N6-(penta-2,3-dienyl)adenine | C10 H11 N5 | 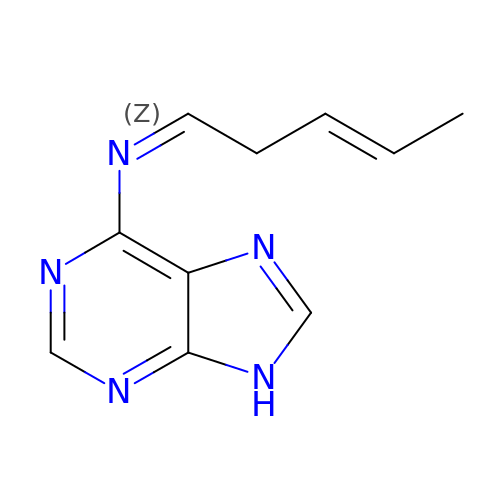ZZNYJUJEPRMVEH-OKBMCRLZSA-N> MARGREAVTLLLVGWGYAPGMQTLEALDAVRRADVVYVESYTMPGSSWLYKSVVEAAGEARVVEASRRDLEERSREIVSRALDAVVAVVTAGDPMVATTHSSLAAEALEAGVAVRYIPGVSGVQAARGATMLSFYRFGGTVTLPGPWRGVTPISVARRIYLNLCAGLHTTALLDVDERGVQLSPGQGVSLLLEADREYAREAGAPALLARLPSVLVEAGAGGGHRVLYWSSLERLSTADV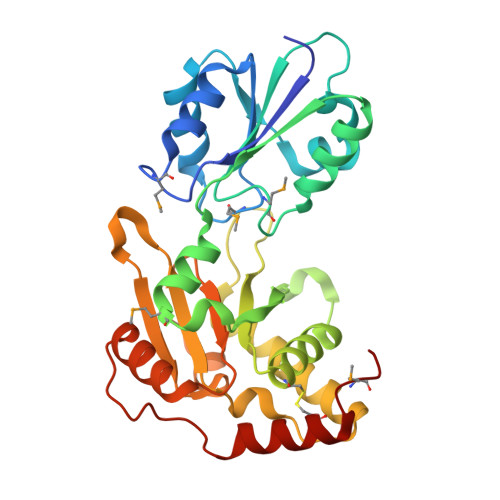EGGVYSIVIPARLSGVEEWLLAAASGQRRPLEYDRSVYETVEENCKKGVYMEPV> LKWIPRNLPSCLINVESSVTSVKLHPNLPIVFVATDHGKLYAFDLFNYTIPLASLQSHTKAITSMDVLFTNYTNSSKKNYLVIVTASKDLQIHVFKWVSEECKFQQIRSLLGHEHIVSAVKIWQKNNDVHIASCSRDQTVKIW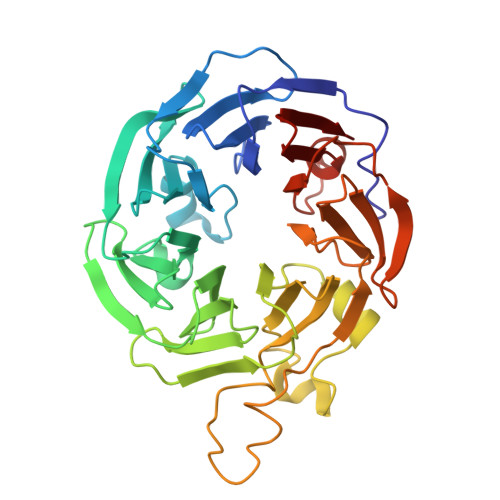DFHNGWSLKTFQPHSQWVRSIDVLGDYIISGSHDTTLRLTHWPSGNGLSVGTGHEFPIEKVKFIHFIEDSPEIRFRTPSTDRYKNWGMQYCVSASRDRTIKIWEIPLPTLMAHRAPIPNPTDSNFRCVLTLKGHLSWVRDISIRGQYLFSCADDKSVRCWDLNTGQCLHVWEKLHTGFVNCLDLDVDFDSNVTPRQMMVTGGLDCKSNVFM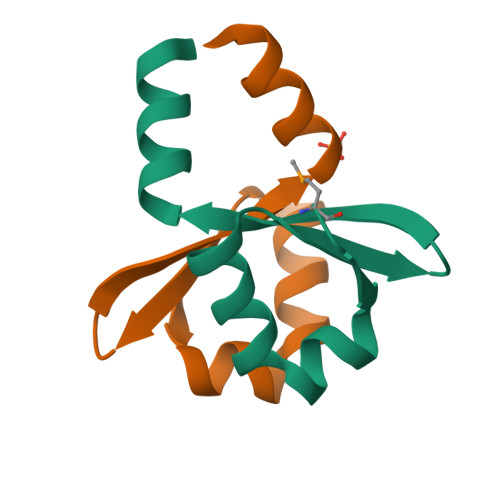>[4x]GHMHVWPVQDAKARFSEFLDACITEGPQIVSRRGAEEAVLVPIGEWRRLQAAARPSLKQLLLSDSARTEMLVPERGKARRRQVEPLRGS> GPHMATGQDRVVALVDMDCFFVQVEQRQNPHLRNKPCAVVQYKSWKGGGIIAVSYEARAFGVTRSMWADDAKKLCPDLLLAQVRESRGKANLTKYREASVEVMEIMSRFAVIERASIDEAYVDLTSAVQERLQKLQGQPISADLLPSTYIEGLPQGPTTAEETVQKEGMRKQGLFQWLDSLQIDNLTSPDLQLTVGAVIVEEMRAAIERETGFQCSAGISHNKVLAKLACGLNKPNRQTLVSHGSVPQLFSQMPIRKIRSLGGKLGASVIEILGIEYMGELTQFTESQLQSHFGE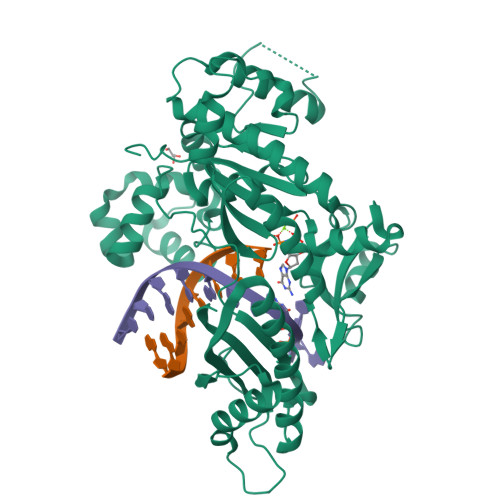KNGSWLYAMCRGIEHDPVKPRQLPKTIGCSKNFPGKTALATREQVQWWLLQLAQELEERLTKDRNDNDRVATQLVVSIRVQGDKRLSSLRRCCALTRYDAHKMSHDAFTVIKNMNTSGIQTEWSPPLTMLFLCATKFSAS Carotenoid cleavage dioxygenases (CCDs) are non-heme FeII enzymes that catalyze the oxidative cleavage of alkene bonds in carotenoids, stilbenoids, and related compounds. pmcCarotenoid cleavage dioxygenases (CCDs) are a broadly distributed superfamily of enzymes that catalyze the reaction of dioxygen (O2) with carotenoids, stilbenoids, and related redox-active polyenes. These enzymes use a mononuclear non-heme FeII center to activate O2 for reaction with a specific alkene group in the substrate, generating carbonyl-containing products of importance in biological processes such as hormonal signaling and light detection. Unlike many mononuclear non-heme iron dioxygenases that coordinate their FeII centers using a 2-His, 1-Glu/Asp “facial triad” motif, CCDs use a 4-His cluster, three of which hydrogen bond to second-sphere carboxylates (Glu/Asp). While one coordination position is occupied by a solvent ligand as demonstrated by several crystallographic and spectroscopic investigations, the other is vacant because of apparent occlusion by a nearby methyl group of a semiconserved, second sphere residue (i.e., Thr/Val/Ile), making CCDs five-coordinate (5C) in their resting FeII states.

To investigate whether reduction in side-chain volume would allow solvent binding at the sixth position, site-directed mutagenesis was used to introduce a T151G substitution in CAO1, thereby opening the maximal potential space for ligand coordination. Globally, the structure of T151G FeII–CAO1 closely resembled the wildtype protein with an overall Cα RMSD of 0.125 Å. Two discrete density map peaks were observed in proximity to the iron center indicating two coordinated solvent molecules. One of these (solvent 1) corresponded to the normally bound water molecule located trans to His197. The second peak, located across from His313, was also satisfactorily modeled with a water molecule (solvent 2). The newly accessible space for solvent coordination was readily apparent in the solvent-excluded surface of the T151G FeII–CAO1 variant. The average Fe–O bond lengths for solvents 1 and 2 were 2.52 ± 0.15 Å and 2.80 ± 0.10 Å, respectively, indicating relatively weak coordination. The ∠His197Nε–Fe–H2O for solvent 1 is 170°, whereas solvent 2 is distorted away from a trans geometry with an ∠His313Nε–Fe–H2O of ∼153°. This distortion arises from the solvent avoiding a steric clash with a nearby Ala196 side chain as well as its engagement in a weak hydrogen bonding interaction with the main chain carbonyl oxygen of residue 151. In the stilbenoid-cleaving CAO1, the volume of the side chain was maximally reduced by making a Thr to Gly substitution.

>[4x]MAEYVFSDAPKDSHGNGVKDAVPGKQPEELPPAPRYFQGENTAGFMRPVRFEGDITNLEVVGEIPKSIEGTFYRVMPEPHLPSFIPNDPWFNGDGNISGFYFKDGHVDLKQRYVRTEKFVREAEARRSLLGKYRNRYTDLVEFKIRSTANGNIVYWRGQLLALKEDSPPYAMDPETLETFGVYDFDGQLPSLTFTAHPKFDPVTREMVCFGYEAKGDGTRDICYYSFGPDGKIAETVWLVSPVCGMIHDFAVTENFVIFPIIPLVCDVERMKQGGDHWQWDYSIPMYIGVLPRRGAQGSDVKWFEAPHGFAGHVANAFEDDKGHIQLQMAYAKDNVFFWWPDANGKGPRPGEVEAHFANFVLDYQSDKLPLAEPTYLVDDDMEFPRIDDRVATRKHKHTFFCIFDRKPGVTDFEFVMPRAGGGAPMSNGLAHLNHETGDIQRYLPGPRKLTGECIFIPRNSEAAEGDGYVMVLLANYEDMCSELAVLDTKDLTNEVALIKLPVRLRPGLHGNWVDKSDVDGHPAPL BCL-2 is the founding member of the pro-survival class of proteins that includes BCL-XL, BCL-W, A1/BFL-1 and MCL-1. They exert their pro-survival function by binding and restraining related members of a family of pro-apoptotic proteins—the sensors of cellular stress (the BH3-only proteins) and the effectors of apoptosis (BAX and BAK). Four or more hydrophobic amino acids on successive helical turns within the BH3 motif engage complementary pockets (P1 through P4) in this surface groove of pro-survival proteins. Venetoclax competes with pro-apoptotic BH3 motifs for BCL-2 binding, releasing pro-apoptotic proteins and allowing apoptosis in cells primed for death.

To predict potential resistance mutants a mouse model was used to induce venetoclax tolerance in cancer cells. This study identified that mutation of phenylalanine 104 (human numbering) to either leucine (F104L) or cysteine (F104C), located within BCL-2’s BH3-binding groove, rendered the lymphoma cell line resistant to venetoclax. The crystals of venetoclax complexed with BCL-2 F104L and BCL-2 WT are isomorphous. Well-defined electron density for the drug in the mutant complex structure suggests two conformations for the 4DM and acyl group of the BA moiety as in WT. The side chain of F104 separates the P2 and P4 pockets of BCL-2. The P4 pocket volume was maintained between WT and F104L structures (P4 pocket volume 380 Å3 for both WT and F104L). In contrast the volume of the P2 pocket increased with the F104L mutation as the leucine sidechain occupies a smaller volume than phenylalanine. In this structure two conformers for F112 on α3 are evident, one like WT and a second occupying some of the volume vacated by the F104L mutation. The new F112 conformation extends into the P2 pocket, packing against L104. The occupancy of F112 refined to 0.48 for the conserved conformation and 0.52 for inserted conformation, indicating that the compensation in P2 pocket volume only occurs 50% of the time and the vacated space is unfavoured. The structure of BCL-2-F104L:venetoclax presented here reveals that the P2 pocket increases in volume with the F104L mutation relative to WT (480 Å3 and 596 Å3 for WT and F104L, respectively). This increase in pocket volume decreases the surface complementarity between the drug and its target, likely contributing to the decrease in affinity.

> MAHAGRTGYDNREIVMKYIHYKLSQRGYEWDAGDDVEENRTEAPEGTESEVVHLTLRQAGDDLSRRYRRDFAEMSSQLHLTPFTARGRFATVVEELFRDGVNWGRIVAFFEFGGVMCVESVNREMSPLVDNIALWMTEYLNRHLHTWIQDNGGWDAFVELYGPSMR>[4x]MGMKLLVVSWGDFERWKETKYRFGGETSVGPSTLPILQKVIKPDWTVIVLSDTIGKDFSSVETLREDVRNRVMDFLDRIGAGREVDVIIAPGIGEFTHGSFRGSAMDAYYYVLHALSEIIPTKGDLEVHFDSTHGLNYVTLLTYRALKDLLGIAAVMNTVTFYAYNSDPFVPKITKELNINT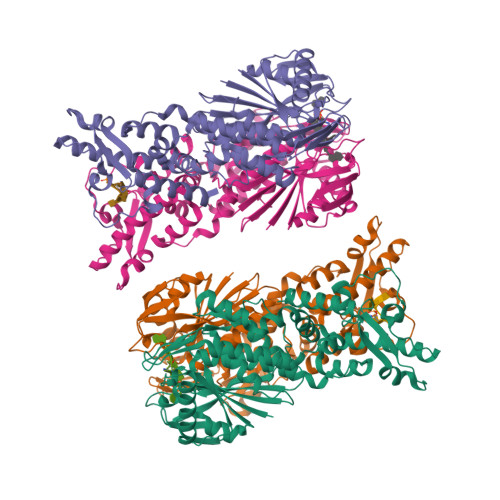IETTMVKPTPLSEPLPGFDEYLCPYSMERAEFVRLKGSLNTLKNLRKEKKKLEAWIGSLLFGLPLLFLEEFPDIGRLESYIEELAETWGGAIAVNAEEKAVTRRLAFGSGFGTLVKLLFQARITRGLLVEEPYSIEKLYSVSDRLFRGSTLQRVRVELGKIEDKAIKYARKGAFPRDIPLRDFLGFDAANREVSPRNVLAHAGLEANVVEVSMEAWEPKRPEEEAGRHTHLKYTPVGLKKVEDIVSRALKESHHHHHH>[12x]MAEREGFAAEGAKAVYDRLKNGRQPYETRAQNCAAVTIPSLFPKESDNSSTEYTTPWQAVGARCLNNLAAKLMLALFPQSPWMRLTVSEYEAKTLSQDSEAAARVDEGLAMVERVLMAYMETNSFRVPLFEALKQLIVSGNCLLYIPEPEQGTYSPMRMYRLVSYVVQRDAFGNILQIVTLDKVAFSALPEDVKSQLNADDYEPDTELEVYTHIYRQDDEYLRYEEVEGIEVA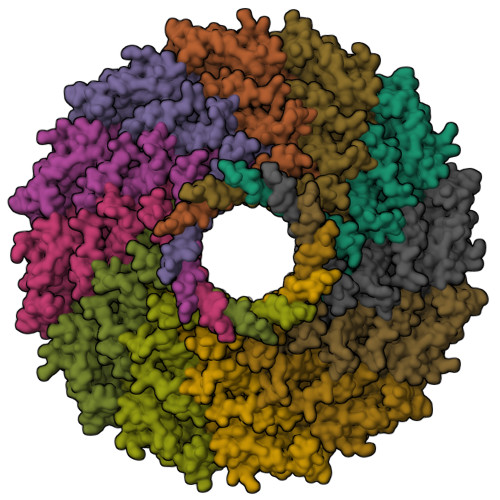GTEGSYPLTACPYIPVRMVRLDGEDYGRSYCEEYLGDLNSLETITEAITKMAKVASKVVGLVNPNGITQPRRLNKAATGEFVAGRVEDINFLQLTKGQDFTIAKSVADAIEQRLGWAFLLNSAVQRNAERVTAEEIRYVAGELEATLGGVYSVQSQELQLPIVRVLMNQLQSAGMIPDLPKEAVEPTVSTGLEALGRGQDLEKLTQAVNMMTGLQPLSQDPDINLPTLKLRLLNALGIDTAGLLLTQDEKIQRMAEQSSQQAVVQGASAAGANMGAAVGQGAGEDMAQA O,O-diethyl O-{4-[(R)-methylsulfinyl]phenyl} 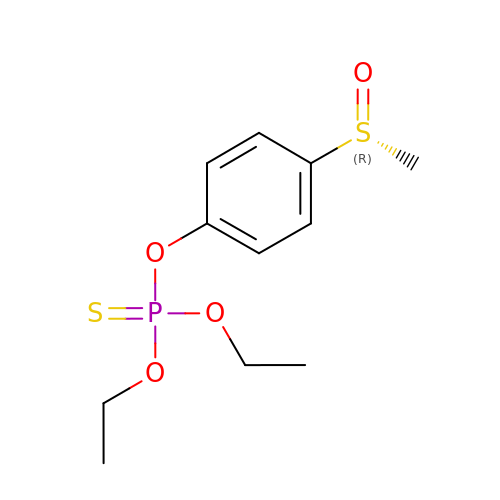phosphorothioate | C11 H17 O4 P S2 | XDNBJTQLKCIJBV-GOSISDBHSA-N>MASAIVLINTDAGGEDEVFERLKSMSEVTEVHVVYGVYDIVVKVEADSMDKLKDFVTNTIRKLPKVRS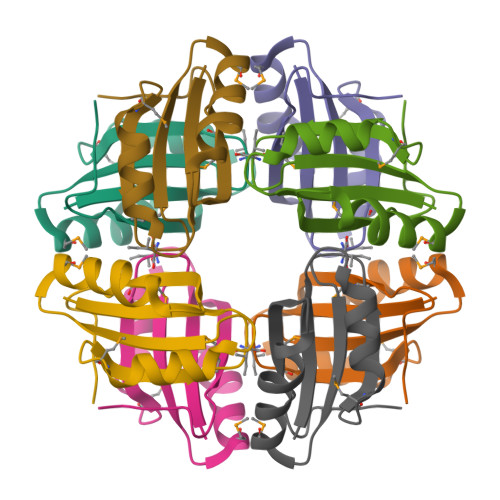TLTMIIVEGKSLVKK[8x]Zaragozic acid A | C35 H46 O14 | 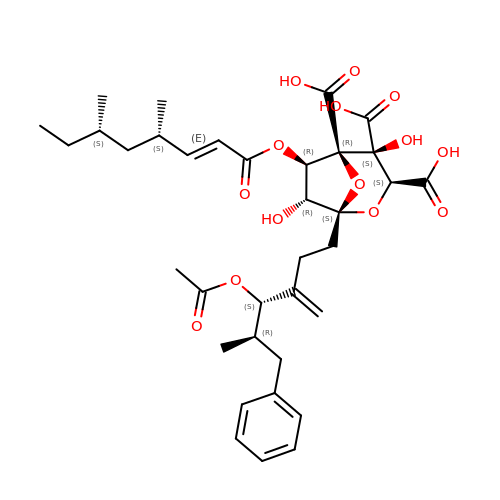DFKDOZMCHOGOBR-NCSQYGPNSA-N>[2x]MSLSIPREFSNAIRFLSIDATLKAKSGHPGMPMGMADIATVLWTKFLKHNPNNPHWINRDRFVLSNGHGSMLLYSLLHLTGYDLSIEDIKNFRQLHSKTPGHPEYGYTPGVETTTGPLGQGVANAVGMALGEKLLSDRYNTPDLKVIDHHTYVFLGDGCLMEGVSHEACSLAGTLGLNKLVAFWDDNNISIDGDTKGWFSDNTPERFRAYGWHVIENVDGHDFVAIEKAINEAHSQQQKPTLICCKTVIGFGSPEKAGTASVHGSPLSDQERASAAKELNWDYQAFEIPQDVYKYWDAREKGQALEANWQGQRNLFKDSPKFDEFERVLSKELPVG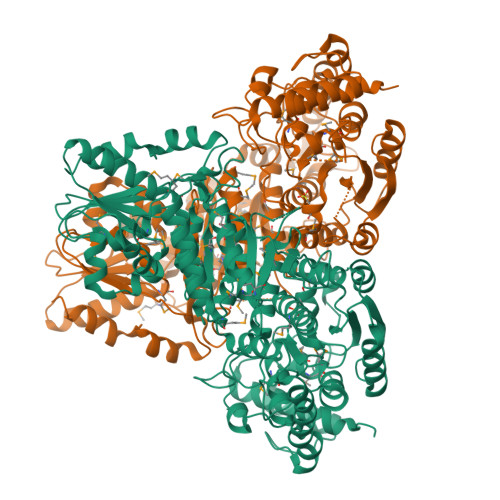LESAINDYIASQLSNPVKVATRKASQMVLEVLCKNMPEMFGGSADLTGSNNTNWSGSVWLNNTQEGANYLSYGVREFGMAAIMNGLSLYGGIKPYGGTFLVFSDYSRNAIRMSALMKQPVVHVMSHDSIGLGEDGPTHQPIEHVPSLRLIPNLSVWRPADTIETMIAWKEAVKSKDTPSVMVLTRQNLMPVVQTQHQVANIARGGYLVKDNPDAKLTIVATGSEVELAVKVANEFEKKGIKLNVASIPCVEVFATQAHEYKKTVIKDDIPAVFVEMAQPDMWYKYMPKAGGEVKGIYSFGESAPAEDLFKRFGFTVENISNIVAKYV2,2-dimethyl-7-(2-oxidanylidene-3~{H}-imidazo[4,5-b]pyridin-1-yl)-1-(phenylmethyl)-3~{H}-quinazolin-4-one | C23 H21 N5 O2 | 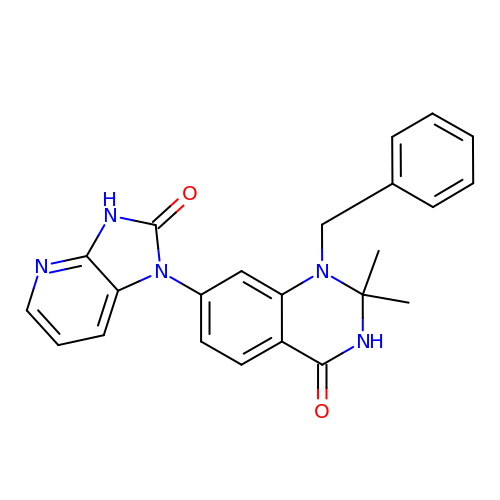LOPPJVYTMBRTCK-UHFFFAOYSA-N In Xenopus eggs, NPM2 replaces sperm protamines with core histones upon fertilization, thereby promoting nucleosome assembly on sperm DNA Laskey et al., 1978; Philpott et al., 1991; Ohsumi and Katagiri, 1991. NPM2 can also extract out somatic linker histones from chromatin Dimitrov and Wolffe, 1996; Ramos et al., 2005; Bañuelos et al., 2007. The acidic tracts in the C-terminal tail of NPM2 binds H2A-H2B, histone octamers, and the linker histone H5 Platonova et al., 2011; Ramos et al., 2010; Taneva et al., 2009, while poly-glutamylation and hyperphosphorylation of NPM2 promote its substrate sequestration ; Lorton et al., 2023. Our cryo-EM structure strongly suggests that the NPM2 binds to H1.8 as a homo-pentamer.

3D DuSTER enabled the reconstruction of 3D structure of the interphase-specific H1.8-containing complex, a pentameric macromolecule with a diameter of approximately 60 Å. C5 symmetry was applied during structural reconstruction. Among the proteins detected by MS, NPM2 aligned well with the MagIC-cryo-EM result. In addition, the crystal structure and AlphaFold2 (AF2)-predicted models of Xenopus NPM2 matched the MagIC-cryo-EM structure of the interphase-specific H1.8-bound complex Dutta et al., 2001. By combining MagIC-cryo-EM and DuSTER, we were able to determine the sub-nanometer structure and structural variations of the NPM2-H1.8-GFP complex, in which the mass of the ordered region is only 60 kDa. One possibility is that the H1.8 structure in NPM2-H1.8 does not follow C5 symmetry. As the size of the NPM2-H1.8 complex estimated from sucrose gradient elution volume is consistent with pentameric NPM2 binding to a single H1.8, applying C5 symmetry during structural reconstruction likely blurred the density of the monomeric H1.8 that binds to the NPM2 pentamer. The structural determination of NPM2-H1.8 without applying C5 symmetry lowered the overall resolution but visualized multiple structural variants of the NPM2 protomer with different degrees of openness co-existing within an NPM2-H1.8 complex, raising a possibility that opening of a portion of the NPM2 pentamer may affect modes of H1.8 binding. While DuSTER enables the structural analysis of NPM2 co-isolated with H1.8-GFP, the resulting map quality is modest, and the reported numerical resolution may be overestimated.

>[5x]MASTVSNTSKLEKPVSLIWGCELNEQNKTFEFKVEDDEEKCEHQLALRTVCLGDKAKDEFHIVEIVTQEEGAEKSVPIATLKPSILPMATMVGIELTPPVTFRLKAGSGPLYISGQHVAMEEDYSWAEEEDEGEAEGEEEEEEEEDQESPPKAVKRPAATKKAGQAKKKLDKEDESSEEDSPTKKGKGAGRGRKPAAKK>[12x]MNTPEHMTAVVQRYVAALN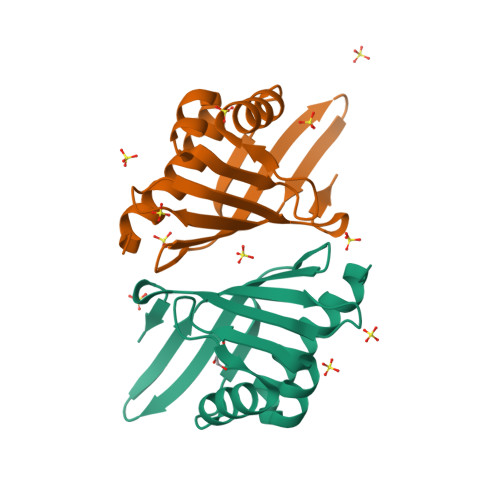AGDLDGIVALFADDATVEEPVGSEPRSGTAAIREFYANSLKLPLAVELTQEVRAVANEAAFAFTVSFEYQGRKTVVAPIDHFRFNGAGKVVSMRALFGEKNIHAGA>[2x]GSTGSMVKSGKARAHTNIALIKYWGKADETYIIPMNNSLSVTLDRFYTETKVTFDPDFTEDCLILNGNEVNAKEKEKIQNYMNIVRDLAGNRLHARIESENYVPTAAGLASSA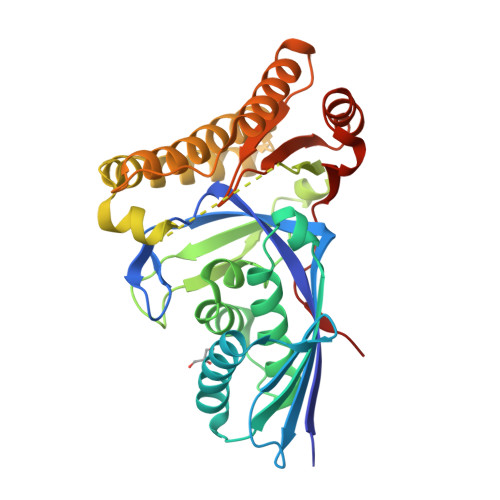SAYAALAAACNEALSLNLSDTDLSRLARRGSGSASRSIFGGFAEWEKGHDDLTSYAHGINSNGWEKDLSMIFVVINNQSKKVSSRSGMSLTRDTSRFYQYWLDHVDEDLNEAKEAVKNQDFQRLGEVIEANGLRMHATNLGAQPPFTYLVQESYDAMAIVEQCRKANLPCYFTMDAGPNVKVLVEKKNKQAVMEQFLKVFDESKIIASDIISSGVEIIK> GSREREAGERRAQNACTLAAVTEKLGRAAELDYCDLEALHAELEPLARSADAAPQVEQFNELLTERARVPRRDLEHELLERRCDTELFVSTDDSVHELREKAGLLFQLSQLLLPEPRADQLWNFVCMANNFRIKFIYHFTSPSAESEQQSIENYFKFLDKYLSENLYKYMDIFEDESKGITRTLIHKQFINHILEPVREKVNVTMTKIAASNSASDVKMLVLLISEIFITDNALKKSHYYDGVGLVSLIDEAALEVWQNFEVESAVSQFEKLTTPGASLMS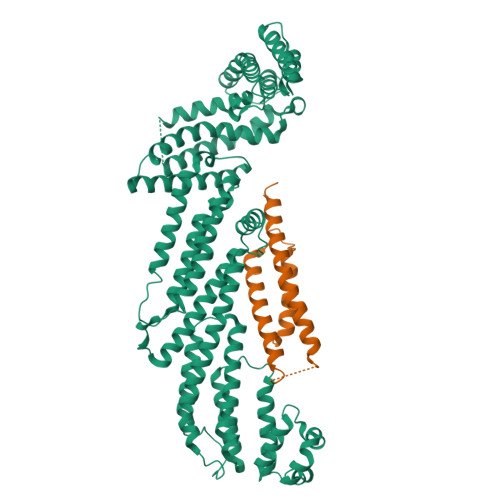PKNGADFGKLLENMYRYLEPFFSIDYRNLFSVKYQLVDEIFIQLPLKYRSFLLSKNILQNELTAEQQFENTCVKLHSLLLISNILVRFSHDFTFIEMTQQINKITDSDYEYIFDEVWESYDEAVIVLRDSIVHRWVKGLSSSLRNYFKYNEWDSIATAPEQCSAELVGALAWMKKMTDIFDKYWYPQHIIAQIKVALLENIIKFMLNYVVKLNKFSENGLRQLTFDYEALRATLGLPLEHSSVAEELALFEYFNILSMKYTNNKITSKFLDAEYVSSHHTRNFRELRESLQVSHLTSDEIADALYRTL;> MGSMPYATQLALLQDELLDMLEPRDGEGLRTADIIDKTLRFRELLGCYRLQVEKSTRQLELPRQVRTAAALRGAHAPASQAPALAQLLLWERFLADYRRRLDAAIVHEHEATAARQLQARPTAARAPRAPMTAKDRLLA>GMGFEEEEVRFRLDDTDKQEISKTLTSVYRSLEEKGYNPINQIIGYVLSGDPAYIPRYNDARNQIRKHERDEIIEELVRYYLKGNGIDL[2x]

Here, we identify a protein (CcpS) that is phosphorylated by Stk1 and modulates the activity of phosphatase CpsB in Streptococcus suis, thus linking Stk1 to CPS synthesis. The crystal structure of CcpS shows an intrinsically disordered region at its N-terminus, including two threonine residues that are phosphorylated by Stk1. The activity of phosphatase CpsB is inhibited when bound to non-phosphorylated CcpS. Thus, CcpS modulates the activity of phosphatase CpsB thereby altering CpsD phosphorylation, which in turn modulates the expression of the Wzx-Wzy pathway and thus CPS production.

To gain more insights into the phosphorylation events of CcpS, we further analyzed the X-ray crystal structure of CcpS-T4ET7E, which mimics the CcpS-P. Although we obtained a high-resolution X-ray crystal structure of CcpS-T4ET7E, we still could not resolve the N-terminal flexible region structure. Superimposition of CcpS onto CcpS-T4ET7E folded structure revealed that overall structure was highly similar to each other; however, we can observe that a resolvable structure of N-terminal partial region is significantly different between CcpS and its variant CcpS-T4ET7E (chain A, N-ter). These results indicated that the highly flexible N-terminal disorder region of CcpS may be not have contributed to intrinsic stability, but was closely related to its binding partners and their functions. Although the electron density map of the N-terminus was not clear, the partially folded structure of the N-terminus between CcpS and CcpS-T4ET7E chain A crystal structure was obviously different (chain A, N-ter). Notably, the ligand CcpS-T4ET7EN has a lower affinity to CpsB than ligand CcpSN. As expected, rCcpS-T4VT7V has a higher affinity to rCpsB and much more than rCcpS-T4ET7E at least tenfold. This result further supported that CcpS phosphorylation indeed modulated the affinity to CpsB. However, rCcpS-P or phospho-mimetic rCcpS-T4ET7E has no significant effect on the process of de-phosphorylation of rCpsD-P catalyzed by rCpsB. The most likely reason for this is that the glutamic acid substitution can not fully mimicked phosphorylation at Thr4 and Thr7 in vivo. Instead, CcpS-T4ET7E possessed properties of both the phosphorylated and non-phosphorylated forms in vivo.>GFQKIPVALLTTTGRKTGQPRVNPLYFLRDGGRVIVAASKGGAEKNPMWYLNLKANPKVQVQIKKEVLDLTARDATDEERAEYWPQLVTMYPSYQDYQSW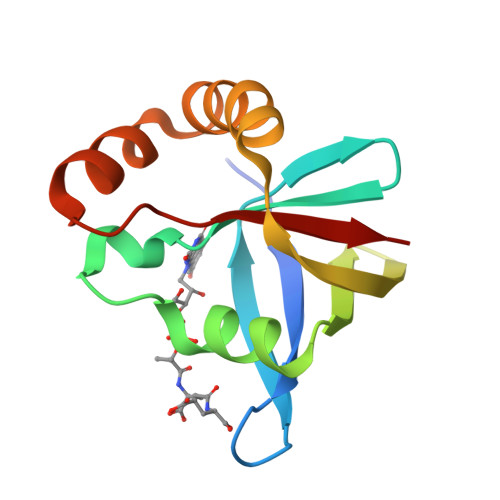TDRTIPIVVCEP[10x]> RDHFALDRPSETHADYLLRTGQVVDISDTIYPRNPAMYCEEARLKSFQNWPDYAHLTPRELASAGLYYTGIGDQVQCFCCGGKLKNWEPCDRAWSEHRRHFPNCFFVLGRNLN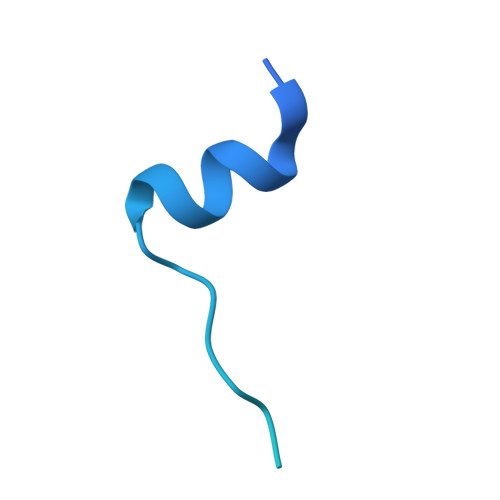IRSESD>MPMFIVNTNVPRASVPDGFLSELTQQLAQATGKPPQYIAVHVVPDQLMAFGGSSEPCALCSLHSIGKIGGAQNRSYS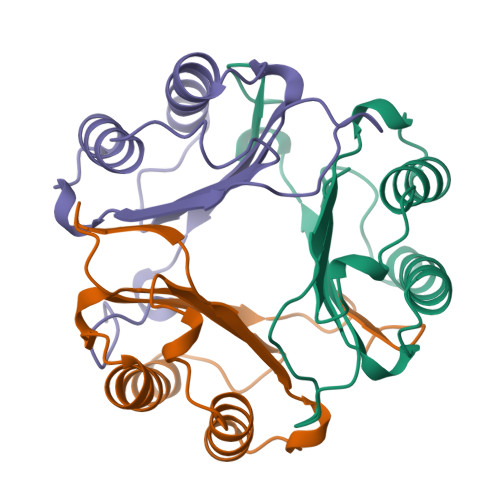KLLCGLLAERLRISPDRVYINYYDMNAASVGWNNSTFA[3x]>[2x]GAMDARSVNGEFPRHVKLKNEIENLLDQVTQLYTKHNSNYQQYNAQAGR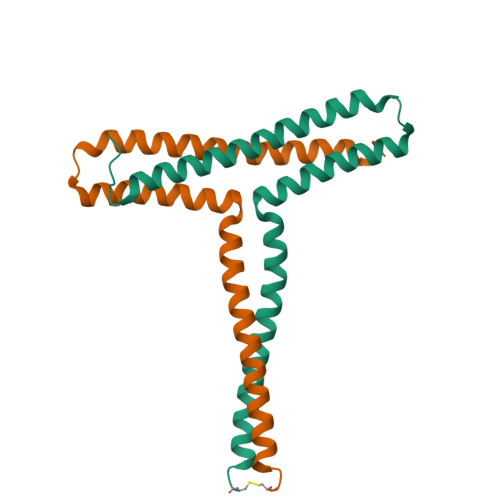LDLRQKAEYLKGLNDWAERLLQELNGEDVKKVLGKVAFEKDDLEKEVKELKEKIDKKEKEYQDC> SMTTPVSPSPSGIIPAQLGFLAIYNPALGTTDETLEDQIVYYATASTLSQARRRHRRPRRRDRQRAQSVVKDSRPNAAGATGDSEAVAEDKD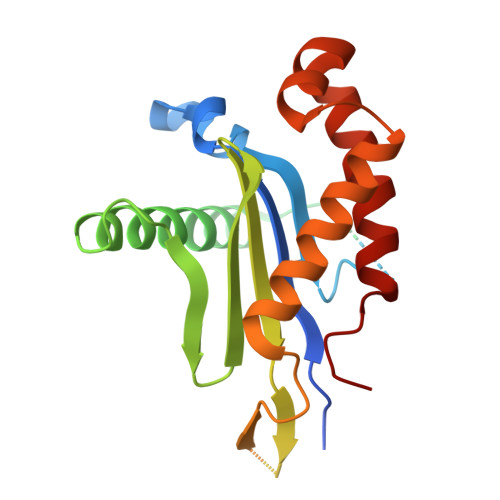PVSKEERHERLRQIGLAQGMVEFAKSFSDGEPVDTIDTEKARVILVEVEEGWWILASIDLTRLPLPQIKTPTSSSAPPPAPNLNPLPPEPAYEYSSREVKPPSLLRADLLRAYDLFLLHHGSSLSSLLASQGRAQLVASLTRFWDHFLATWNVLLHGN The E3 ubiquitin ligase HERC2 has been linked to neurological diseases and cancer, however it remains a poorly characterized human protein. The HERC2 gene encodes a large, 4834 residue protein that in addition to the ZZ domain contains three RCC1-like domains (RLDs), a cytochrome b5-like motif (Cyt b5), a mind-bomb/HERC2 (M-H) domain, a CPH domain, a DOC domain (HERC2DOC), and the carboxy-terminal catalytic E3 ubiquitin ligase HECT domain. The selectivity of ubiquitination relies on E3, which recognizes a specific degradation signal in the substrate and accelerates the transfer of Ub from E2 to a lysine residue of this substrate. Our findings suggest a role of cytosolic HERC2 in the ubiquitin-dependent degradation pathways.

HERC2ZZ is followed by HERC2DOC of unknown structure and function. To characterize HERC2DOC, we crystallized this domain and determined its crystal structure, refining it to a 2 Å resolution. The HERC2DOC structure consists of nine antiparallel β-strands and two short α-helices. The core of the domain folds into a β-sandwich with the five strands, β2, β3, β8, β5 and β6 forming one β-sheet that packs against another β-sheet containing the four strands, β1, β9, β4 and β7. The first α-helix links β1 and β2 strands and another α-helix, α2, is located between β2 and β3 strands. One of the open ends of the sandwich is delineated by the short loops connecting the β strands, whereas the opposite end is surrounded by the longer loops (bottom and top, respectively). Electrostatic surface potential of HERC2DOC reveals a well-defined negatively charged groove that lays parallel to the β9 strand and is ideally positioned for pairing with an additional positively charged β-strand of a ligand. Because histone H3 regions are highly positively charged and are known to adopt the β-strand conformation in several complexes, we tested whether HERC2DOC can bind any of the H3 regions using a pull-down assay. HERC2DOC does not recognize any of the H3 peptides tested, or other potential ligands, including SUMO1, Ub and the D-box region of CCNB1. The structure of the DOC domain (originally referred to as the APC10 domain) of the protein APC10 superimposes with the structure of HERC2DOC with an r.m.s.d. of 0.9 Å. The binding affinity of HERC2ZZ to the REEE peptide in the presence of HERC2DOC remained unchanged (Kd of 1 µM). We concluded that although HERC2DOC and HERC2ZZ do not appreciably interact, a conformational rearrangement in the protein may occur when the two domains are linked.

> MHHHHHHSSGRENLYFQGFCGRSGKQLKRCHSSQPGMLLDSWSRMVKSLNVSSSVNQASRLIDGSEPCWQSSGSQGKHWIRLEIFPDVLVHRLKMIVDPADSSYMPSLVVVSGGNSLNNLIELKTININPSDTTVPLLNDCTEYHRYIEIAIKQCRSSGIDCKIHGLILLGRIR>AMGAAELRFCNQTIKELMSKKHYNYNFPFLAPVDTVALNIPNYNEIVKQPMDLGTIQSKLANNEYENADDFEKDVRLVF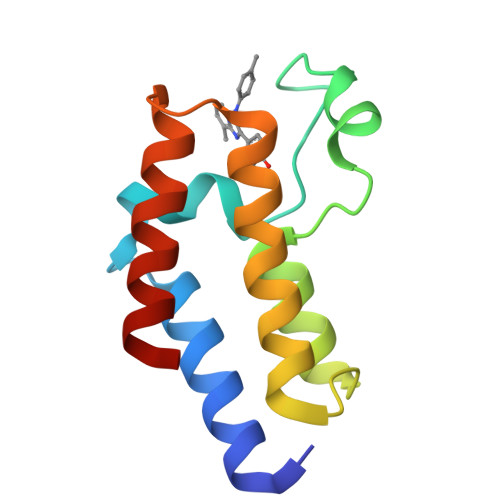KNCYLFNPEGTDVNMMGHRLEAVFDKKWAN[2x]> DPMDLHMMNCELLATCSALGYLEGDTYHKEPDCLESVKDLIRYLRHEDETRDVRQQLGAAQILQSDLLPILTQHHQDKPLFDAVIRLMVNLTQPALLCFGNLPKEPSFRHHFLQVLTYLQAYKEAFASEKAFGVLSETLYELLQLGWEERQEEDNLLIERILLLVRNILHVPADLDQEKKIDDDASAHDQLLWAIHLSGLDDLLLFLASSSAEEQWSLHVLEIVSLMFRDQNPEQLAGVGGSTGSTQRRSALNVRLFLRDFCSEFLENCYNRLMGSVKDHLLREKAQQHDETYYMWALAFFMAFNRAASFRPGLVSETLSVRTFHFIEQNLTNYYEMMLTDRKEAASWARRMHLALKAYQELLATVNEMDISPDEAVRE

Human Timeless is involved in replication fork stabilization, S-phase checkpoint activation and establishment of sister chromatid cohesion. In the cell, Timeless forms a constitutive heterodimeric complex with Tipin. Human Timeless is a large, multi-domain protein of 1208 amino acids. During DNA replication, the Timeless–Tipin complex is part of a larger functional assembly known as the replication pausing (or protection) complex (RPC) that includes Claspin and AND-1 (Mrc1 and Ctf4 in budding yeast, respectively).

In a systematic effort to identify regions of the protein that could be amenable to crystallization, we produced a construct of Timeless spanning residues 1–463, that was highly overexpressed and soluble in recombinant form. Inspection of the 2.2 Å structure revealed that a large segment of the protein construct, spanning residues 239–330, was not visible in the electron density map, presumably because of conformational disorder. Consequently, a new TimN construct was prepared carrying an internal deletion of residues 239–330, that crystallized more readily and yielded crystals diffracting to a higher resolution of 1.85 Å. Removal of residues 239–330 did not cause structural alterations in either the TimN crystal structure, or the solution shape of the Timeless–Tipin complex; small-angle X-ray scattering analysis showed a small but significant decrease in hydrodynamic radius for the complex missing Timeless residues 239–330, indicating that these amino acids are disordered in solution. The N-terminal domain of Timeless is an α-helical protein with an overall shape that is reminiscent of a horseshoe. Although it is not possible to assign TimN to one of the well-known classes of helical-repeat proteins such as the HEAT or ARM repeat families, TimN does contain six two-helix hairpins, with the N-terminal four hairpins containing an additional helix in the intervening segment between the first and the second helix of the hairpin. Surprisingly, TimN forms a dimer in solution and in the crystal; however, SEC multi-angle laser scattering (SEC-MALLS) experiments showed that full-length Timeless exists as a monomer in solution. It is likely therefore that the observed dimerization of recombinant TimN is an artifact of construct design. The peculiar shape of the TimN structure suggests that its concave surface might act as a site of protein–protein interactions.dolichol-phosphate 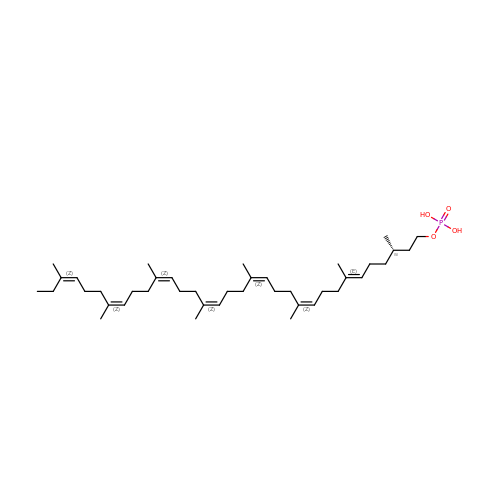(n=4) | C41 H71 O4 P | CMOQFVWDXXQTMI-PJJFLQJDSA-N>DTLESIDNCAVGCPTGGSSNVSIVRHAYTLNNNSTTKFANWVAYHITKDTPASGKTRNWKTDPALNPADTLAPADYTGANAALKVDRGHQAPLASLAGVSDWESLNYLSNITPQKSDLNQGAWARLEDQERKLIDRADISSVYTVTGPLYERDMGKLP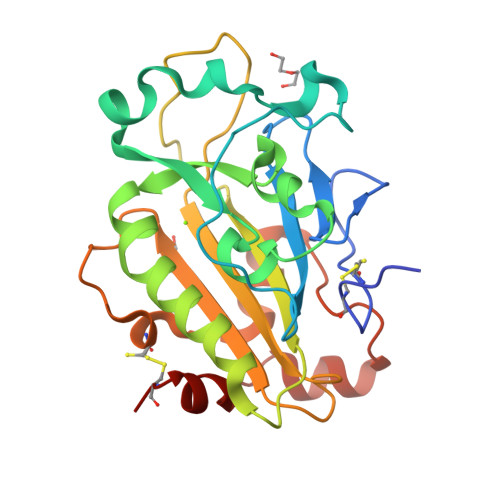GTQKAHTIPSAYWKVIFINNSPAVNHYAAFLFDQNTPKGADFCQFRVTVDEIEKRTGLIIWAGLPDDVQASLKSKPGVLPELMGCKN[2x]Infection by its etiological agent, PRRS virus (PRRSV), shows a highly restricted tropism of host cells and has been demonstrated to be mediated by an essential scavenger receptor (SR) CD163. CD163 fifth SR cysteine-rich domain (SRCR5) is further proven to play a crucial role during viral infection. In the current study, we prepared recombinant monkey CD163 (moCD163) SRCR5 and human CD163-like homolog (hCD163L1) SRCR8, and determined their crystal structures. After comparison with the previously reported crystal structure of porcine CD163 (pCD163) SRCR5, these structures showed almost identical structural folds but significantly different surface electrostatic potentials.

In this work, we prepared recombinant moCD163 SRCR5 in Pichia pastoris X-33 and hCD163L1 SRCR8 in Drosophila melanogaster Schneider 2 (S2) cells, respectively. The recombinant moCD163 SRCR5 and hCD163L1 SRCR8 were eluted as monomer during purification. Their crystal structures were determined and refined to 1.58 Å in P1 space group and 2.0 Å in C2 space group, respectively. MoCD163 SRCR5 was comprised of two antiparallel β-sheets (β1-4, β7 and β5-6) and three helices (a single α-helix α2 and two 310-helices α1, α3), whereas hCD163L1 SRCR8 contained two antiparallel β-sheets (β1-4, β7 and β5-6) and two helices (a single α-helix α1 and a 310-helix α2). A close comparison of moCD163 SRCR5 or hCD163L1 SRCR8 with pCD163 SRCR5 revealed that they shared almost identical structural folds (RMSD = 0.355 Å for 79 matching Cα atoms between moCD163 SRCR5 and pCD163 SRCR5, RMSD = 0.249 Å for 95 matching Cα atoms between hCD163L1 SRCR8 and pCD163 SRCR5). The minor differences between moCD163 SRCR5 and pCD163 SRCR5 were only observed in the long loop regions. MoCD163 SRCR5 displayed a similar surface electrostatic potential as pCD163 SRCR5 did, so-called “D/E-R-rich” charge distribution. The comparison provided a structural basis to explain why stable expression of moCD163 rendered comparable infectivity to PRRSV as pCD163 did, since their crucial SRCR5 shared the overall conformations and surface electrostatic potentials.

>[2x]LEKRPRLVGGDIPCSGRVEVKHGDTWGSVCDSDFSLEAASVLCRELQCGTVVSILGGAHFGEGNGQIWTEEFQCEGHESHLSLCPVAPRPEGTCSHSRDVGVVCSVD> RR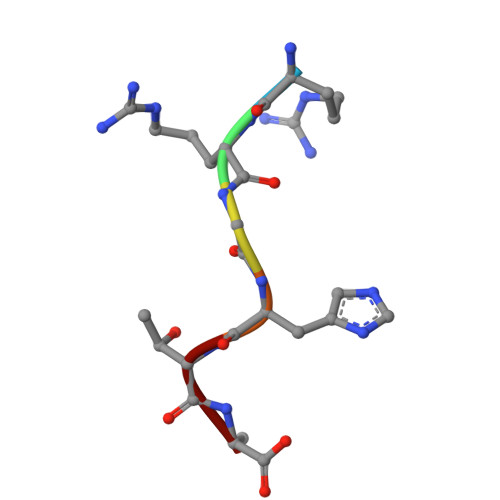GHTA>[2x]MSVHATDAKPPGPSPADQLLDGLNPQQRQAVVHEGSPLLIVAGAGSGKTAVLTRRIAYLMAARGVGVGQILAITFTNKAAAEMRERVVGLVGEKARYMWVSTFHSTCVRILRNQAALIEGLNSNFSIYDADDSRRLLQMVGRDLGLDIKRYSPRLLANAISNLKNELIDPHQALAGLTEDSDDLARAVASVYDEYQRRLRAANALDFDDLIGETVAVLQAFPQIAQYYRRRFRHVLVDEYQDTNHAQYVLVRELVGRDSNDGIPPGELCVVGDADQSIYAFRGATIRNIEDFERDYPDTRTILLEQNYRSTQNILSAANSVIARNAGRREKRLWTDAGAGELIVGYVADNEHDEARFVAEEIDALAEGSEITYNDVAV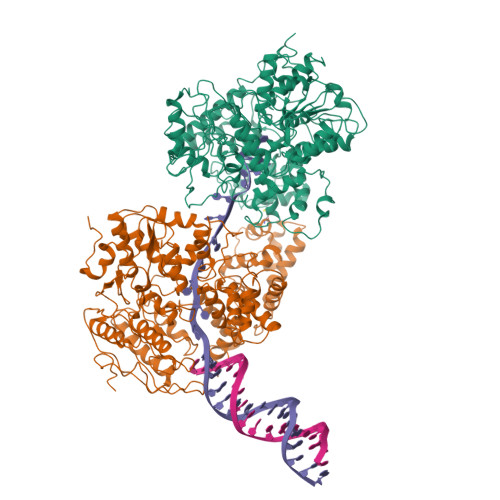FYRTNNSSRSLEEVLIRAGIPYKVVGGVRFYERKEIRDIVAYLRVLDNPGDAVSLRRILNTPRRGIGDRAEACVAVYAENTGVGFGDALVAAAQGKVPMLNTRAEKAIAGFVEMFDELRGRLDDDLGELVEAVLERTGYRRELEASTDPQELARLDNLNELVSVAHEFSTDRENAAALGPDDEDVPDTGVLADFLERVSLVADADEIPEHGAGVVTLMTLHTAKGLEFPVVFVTGWEDGMFPHMRALDNPTELSEERRLAYVGITRARQRLYVSRAIVRSSWGQPMLNPESRFLREIPQELIDWRRTAPKPSFSAPVSGAGRFGSARPSPTRSGASRRPLLVLQVGDRVTHDKYGLGRVEEVSGVGESAMSLIDFGSSGRVKLMHNHAPVTKL>[9x]SNAMMTTAEQIPFQLILNSGNARSFAMEALQFAKQGKMAEADEAMVKAK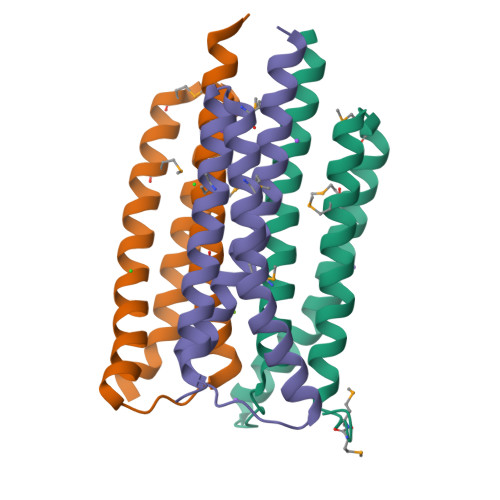EAINEAHHFQTELIQSEARGEKTEISVLLIHAQDHLMNAITVKELAAEFIDLYKKLEAKG> MLQVDIGSTSGKAGSVVSVPITFTNVPKSGIYALSFRTNFDPQKVTVASIDAGSLIENASDFTTYYNNENGFASMTFEA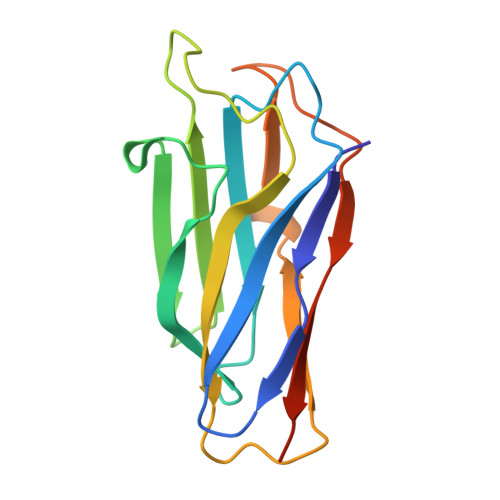PVDRARIIDSDGVFATINFKVSDSAKVGELYNITTNSAYTSFYYSGTDEIKNVVYNDGKIEVIALEHHHHHH geranylgeranyl dihydroxybenzoate 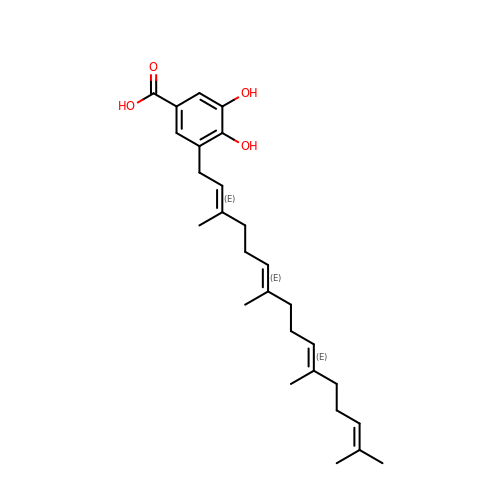| C27 H38 O4 | BSKXNBAQBKFMLO-FLPKSHQQSA-N> MGPCDIYEAGDTPC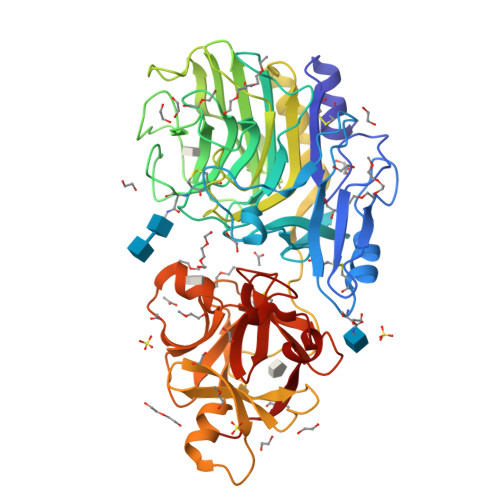VAAHSTTRALYSSFSGALYQLQRGSDDTTTTISPLTAGGIADASAQDTFCANTTCLITIIYDQSGNGNHLTQAPPGGFDGPDTDGYDNLASAIGAPVTLNGQKAYGVFMSPGTGYRNNEATGTATGDEAEGMYAVLDGTHYNDACCFDYGNAETSSTDTGAGHMEAIYLGNSTTWGYGAGDGPWIMVDMQNNLFSGADEGYNSGDPSISYRFVTAAVKGGADKWAIRGANAASGSLSTYYSGARPDYSGYNPMSKEGAIILGIGGDNSNGAQGTFYEGVMTSGYPSDDTENSVQENIVAAKYVVGSLVSGPSFTSGEVVSLRVTTPGYTTRYIAHTDTTVNTQVVDDDSSTTLKEEASWTVVTGLANSQCFSFESVDTPGSYIRHYNFELLLNANDGTKQFHEDATFCPQAALNGEGTSLRSWSYPTRYFRHYENVLYAASNGGVQTFDSKTSFNNDVSFEIETAFAS> GSHMSNTQTVLPFTGLNKPSGVAVDSAGTVYVTDHGNNRVVKLAAGSNTQTVLPFTGLNTPSGVAVDSAGTVWVTDHGNNRVVKLAAGSNTQTVLPFTGLNKPSGVAVDSAGTVYVTDHGNNRVVKLAAGSNTQTVLPFTGLNTPSGVAVDSAGTVWVTDHGNNRVVKLAAGSNTQTVLPFTGLNKPSGVAVDSAGTVYVTDHGNNRVVKLAAGSNTQTVLPFTGLNTPSGVAVDSA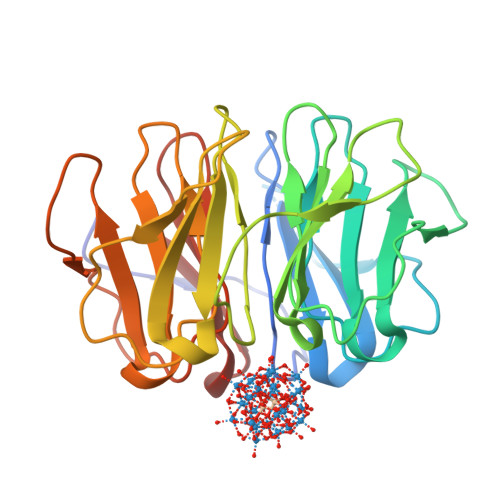GTVWVTDHGNNRVVKLAAG> MAQGNNYGQTSNGVADESPNMLVYRKMEDVIARMQD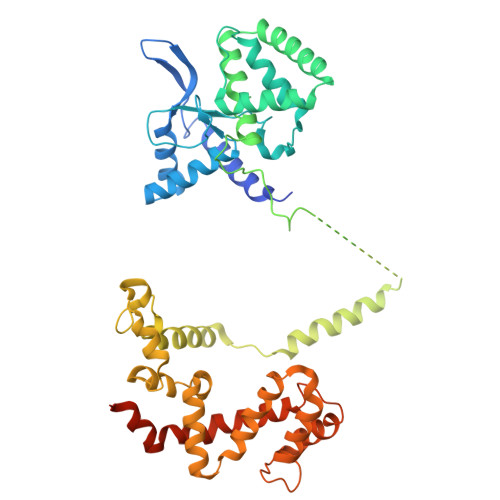EKNGIPIRTVKSFLSKIPSVFSGSDIVQWLIKNLTIEDPVEALHLGTLMAAHGYFFPISDHVLTLKDDGTFYRFQTPYFWPSNCWEPENTDYAVYLCKRTMQNKARLELADYEAESLARLQRAFARKWEFIFMQAEAQAKVDKKRDKIERKILDSQERAFWDVHRPVPGCVNTTEVDIKKSSRMRNPHKTRKSVYGLQNDIRSHSPTHTPTPETKPPTEDELQQQIKYWQIQLDRHRLKMSKVADSLLSYTEQYLEYDPFLLPPDPSNPWLSDDTTFWELEASKEPSQQRVKRWGFGMDEALKDPVGREQFLKFLESEFSSENLRFWLAVEDLKKRPIKEVPSRVQEIWQEFLAPGAPSAINLDSKSYDKTTQNVKEPGRYTFEDAQEHIYKLMKSDSYPRFIRSSAYQELLQAKKKGKSLTSKRLTSLAQSY> STRFTEEYQLFEELGKGAFSVVRRCVKVLAGQEYAAMIINTKKLSARDHQKLEREARICRLLKHPNIVRLHDSISEEGHHYLIFDLVTGGELFEDIVAREYYSEADASHCIQQILEAVLHCHQMGVVHRNLKPENLLLASKLKGAAVKLADFGLAIEVEGEQQAWFGFAGTPGYLSPEVLRKDPYGKPVDLWACGVILYILLVGYPPFWDEDQHRLYQQIKAGAYDFPSPE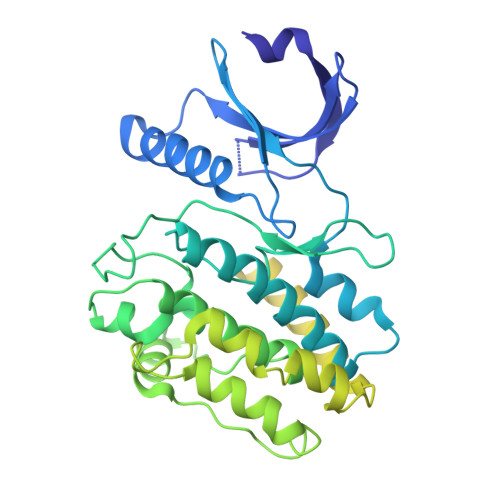WDTVTPEAKDLINKMLTINPSKRITAAEALKHPWISHRSTVASCMHRQETVDCLKKFNARRKLKGAILTTMLATRNFSGGKSGGNKKSDGVKESSESTNTTIEDEDTKVRKQEIIKVTEQLIEAISNGDFESYTKMCDPGMTAFEPEALGNLVEGLDFHRFYFENLWSRNSKPVHTTILNPHIHLMGDESACIAYIRITQYLDAGGIPRTAQSEETRVWHRRDGKWQIVHFHRSGAPSVLPH> HMASMKKKGSVVIVGRINLSGDTAYAQQTRGEEGCQETSQTGRDKNQVEGEVQIVSTATQTFLATSINGVLWTVYHGAGTRTIASPKGPVTQMYTNVDKDLVGWQAPQGSRSLTPCTCGSSDLYLVTRHADVIPVRRRGDSRGSLLSPRPISYLKGSSGGPLLCPAGHAVGIFRAAVSTRGVAKAVDFI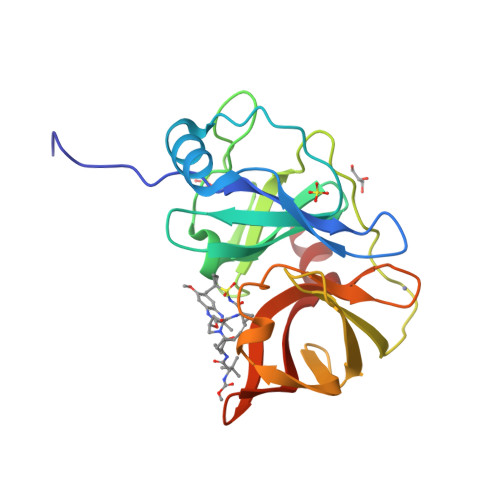PVESLETTMR>[2x]AYTTFSATKNDQLKEPMFFGQPVQVARYDQQKYDIFEKLIEKQLSFFWRPEEVDVSRDRIDYQALPEHEKHIFISNLKYQTLLDSIQGRSPNVALLPLISIPELETWVETWAFSETIHSRSYTHIIRNIVNDPSVVFDDIVTNEQIQKRAEGISSYYDELIEMTSYWH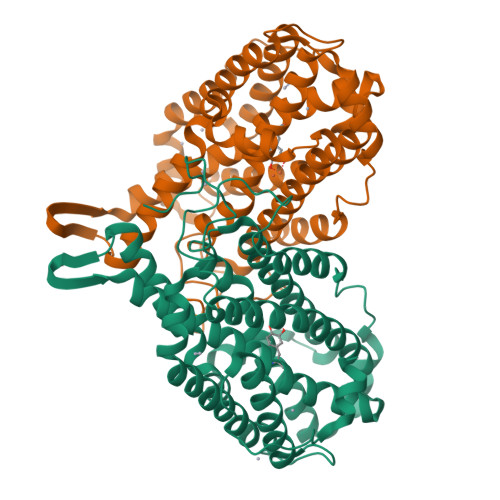LLGEGTHTVNGKTVTVSLRELKKKLYLCLMSVNALEAIRYYVSFACSFAFAERELMEGNAKIIRLIARDEALHLTGTQHMLNLLRSGADDPEMAEIAEECKQECYDLFVQAAQQEKDWADYLFRDGSMIGLNKDILCQYVEYITNIRMQAVGLDLPFNTRSNPIPWINTWLVSDNVQVAPQEVEVSSYLVGQIDSEVDTDDLSNFQL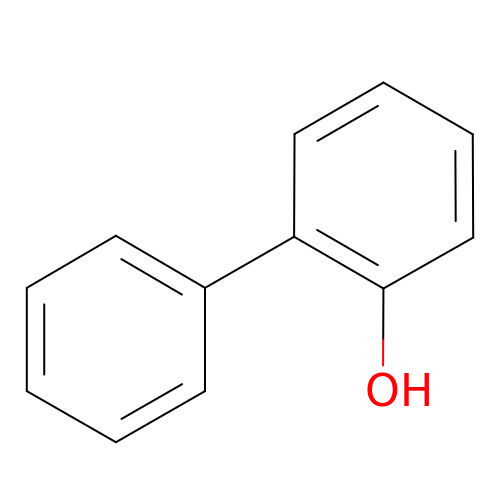2-HYDROXYBIPHENYL | C12 H10 O | LLEMOWNGBBNAJR-UHFFFAOYSA-N>[8x]GDPVTTGKPNILIIMVDQLNGKLFPDGPADFLHAPNLKALAKRSARFHNNYTSSPLCAPARASFMAGQLPSRTRVYDNAAEYQSSIPTYAHHLRRAGYYTALSGKMHFVGPDQLHGFEERLTTDIYPADFGWTPDYRKPGERIDWWYHNLGSVTGAGVAEITNQMEYDDEVAFLANQKLYQLSRENDDESRRPWCLTVSFTHPHDPYVARRKFWDLYEDCEHLTPEVGAIPLDEQDPHSQRIMLSCDYQNFDVTEENVRRSRRAYFANISYLDEKVGELIDTLTRTRMLDDTLILFCSDHGDMLGERGLWFKMNFFEGSARVPLMIAGPGIAPGLHLTPTSNLDVTPTLADLAGISLEEVRPWTDGVSLVPMVNGVERTEPVLMEYAAEASYAPLVAIREGKWKYVYCALDPEQLFDLEADPLELTNLAENPRGPVDQATLTAFRDMRAAHWDMEAFDAAVRESQARRWVVYEALRNGAYYPWDHQPLQKASERYMRNHMNLDTLEESKRYPRGE

The only microbial sulfatases currently assumed to be specific toward one particular substrate are the choline sulfatases (CSs). CSs enable bacteria to use choline-O-sulfate as a source of sulfur, carbon and nitrogen. Based on sequence homology analysis, S. meliloti CS (SmCS) was identified as a member of the AP superfamily and is most closely related to class I ASs. SmCS-catalyzed turnover of choline-O-sulfate in the presence of H218O showed no incorporation of the 18O label in the choline product, indicating that SmCS hydrolyzes choline-O-sulfate via S–O cleavage, thus employing a class I mechanism.

In order to understand the determinants of substrate specificity and catalytic mechanism, we crystallized SmCS and determined its three-dimensional structure by molecular replacement and refined the structure to 2.79-Å resolution. The enzyme crystallizes with eight molecules in the asymmetric unit, and analysis of the structure using the PISA server suggests that the protein is tetrameric with each of the protomers containing two oligomerization interfaces of ~ 2800 and ~ 1600 Å2. The protomer structure of SmCS shows a globular protein with an α/β fold, a central β-sheet surrounded by α-helices, characteristic to proteins in the AP superfamily, confirming that SmCS is indeed a member of this superfamily. The most noticeable structural differences between subgroups within the AP-type ASs and PMHs are in their C-termini, which differ in both length and sequence. In the case of SmCS, the C-terminal tail folds almost around the whole protomer and contains three α-helices that mediate oligomerization (for more details see below). Well-defined and continuous electron density was observed for the active site residues (Asp14, Cys54 and His297) that tetrahedrally coordinated a metal ion. This metal was thus refined as Ca2 +, because it predominated in microPIXE experiments, presumably reflecting its high concentration in the 2 × YT medium, and this was the metal ion used for modeling the crystal structure. Additional positive density was observed in the vicinity of Cys54, suggesting that the latter was partially converted into fGly during production in E. coli. Given that the exact level of fGly conversion is unknown, the structure was modeled with both cysteine and formyl glycine in this position, giving them each 50% occupancy. The active site is closed in this SmCS structure, and the loops that cover the entrance would need to move to allow the subtrate to enter and the products to leave. A hydrogen bond between Asp500 and Asn146 seems to act as a latch that stabilizes the closed conformation.> MQQAPTADQLVKGKNPKLLVLSQRPIVLETPYDLLVSQPERTPKEILYIRNNVDLPGYNTVEGASLDGWKVEVGGLVDKPFTFEAKELLELPQHEVTMVLQCSGNGRSLFQPRTSGN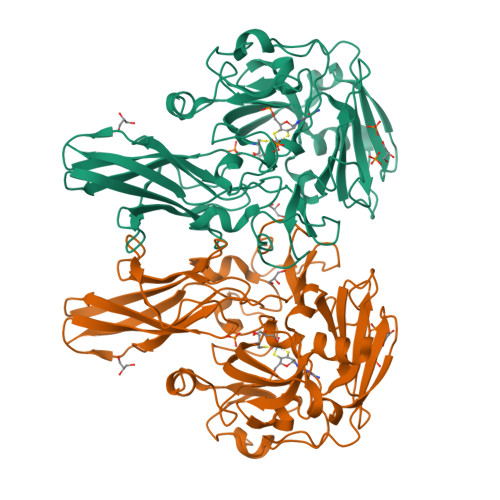PWKRGGVGNVTFRGVRLKDLLEAKGVKLGEKALYITAHASRQGNAPEFVRSVPIHALGHALLALSMNGEPLPAVHGGPIRLVFPGYFGVNNVKWVQKIEFTEAENTTAEQMPRYRVPAIPNANIPFLPQEPGKTYPYSFTNSRPNWLVAINSFIFAPLEGQTVEGPYVRVEGVAFNDGIVPLVSVEVSANGGRTWQQARLERQEKSFGWVRWQATLYLRPGEHEVMARAWDAVGRSQPLDGNIAWNERGYEYNGVMRVKFTVAHHHHHH>[2x]ATVSEVISYWRGLADTGQGYDADLAWGWQCADVTNGTTTNFFGVTLWGNAIDLLD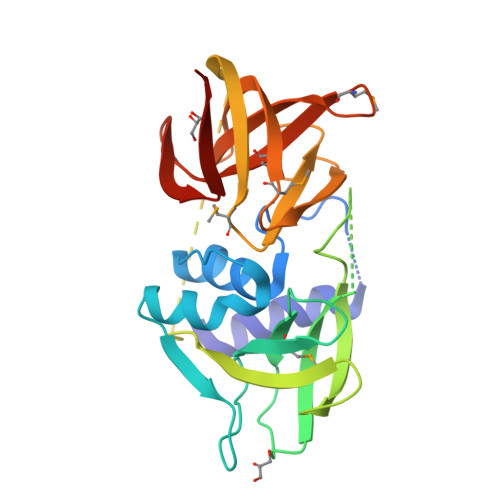SAKAQGLEVIYDAPGINPKAGDLFVMFTYGHPYGHTGIIIADSDGYTIQTIEQNVDGYSDNNGDGINDQFQVGGPARYVTRAFSDGDGYIVGWIRPPYSDTSSEKQSQSQAPSGFRKLKDEVGTFEVMVPALNVRREPSLNGEIVACYQYGMTGTYDSVYVGDGYIWVSYVGASGMRNYMAVGDADGDYNVNPYCKFYLEHHHHHH> PTTCTNCFTQTTPLWRRNPEGQPL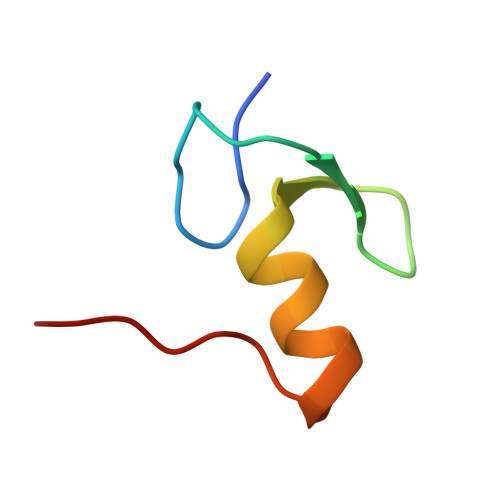CNACGLFLKLHGVVRPLSL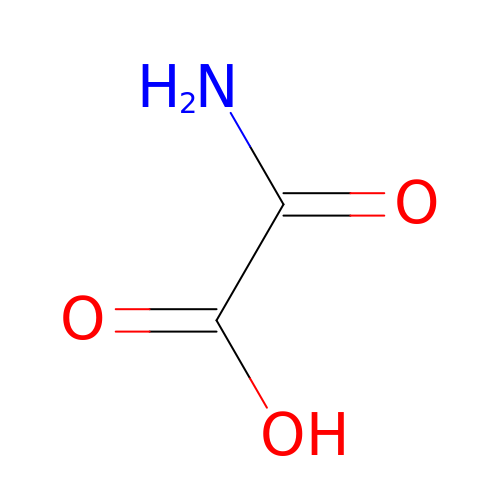OXAMIC ACID | C2 H3 N O3 | SOWBFZRMHSNYGE-UHFFFAOYSA-N>ACPLEKALDVMVSTFHKYSGKEGDKFKLNKSELKELLTRELPSFLGKRTDEAAFQKLMSNLDSNRDN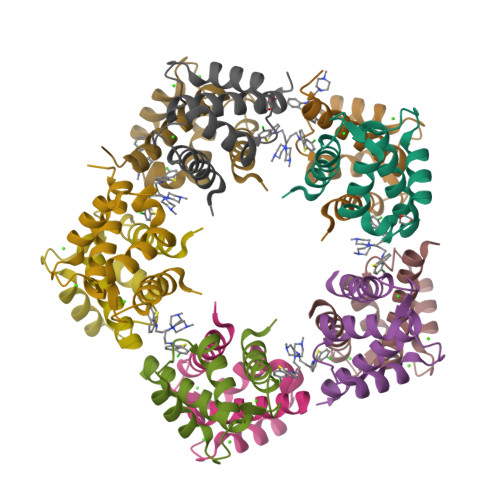EVDFQEYCVFLSCIAMMCNEFFEGFPDKQPRKK[10x]>GSMAPITAYSQQTRGLLGCIITSLTGRDKNQVDGEVQVLSTATQSFLATCVNGVCWTVYHGAGSKTLAGPKGPITQMYTNVDQDLVGWPAPPGARSMTPCTCGSSDLYLVTRHADVIPVRRRGDSRGSLLSPRPVSYLKGSSGGPLLCPSGHVVGIFRAAVCTRGVAKAVDFIPVESMETTMRSPVFT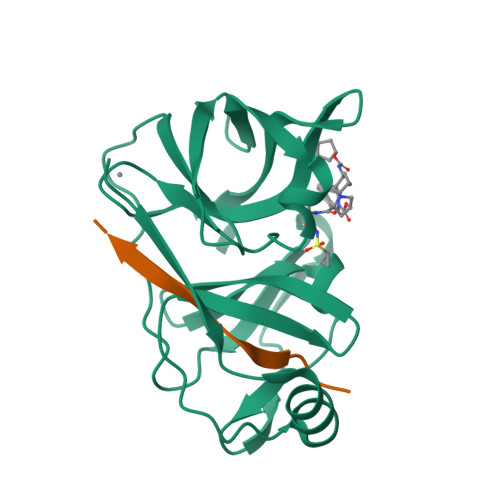DN[2x];>KGSVVIVGRIILSGRK[2x]> MPNPDNTEAYVAGEVEIENSAIALSGIVSVANNADNRLEVFGVSTDSAVWHNWQTAPLPNSSWAGWNKFNGVVTSKPAVHRNSDGRLEVFVRGTDNALWHNWQTAADTNTWSSWQPLYGGITSNPEVCLNSDGRLEVFVRGSDNALWHIWQTAAHTNSWSNWKSLGGTLTSNPAAHLNADGRIEVFARGADNALWHIWQTAAHTDQWSNWQSLKSVITSDP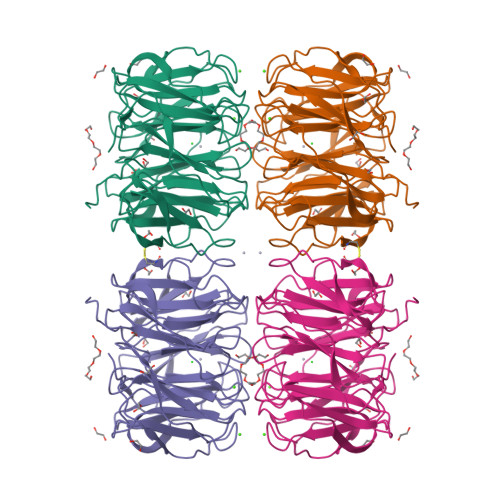VVINNCDGRLEVFARGADSTLRHISQIGSDSVSWSNWQCLDGVITSAPAAVKNISGQLEVFARGADNTLWRTWQTSHNGPWSNWSSFTGIIASAPTVAKNSDGRIEVFVLGLDKALWHLWQTTSSTTSSWTTWALIGGITLIDASVIK> MRVVIVGGGFGGIAAASQLKSWAVPFVLVDMRDAFHHNVAALRASVESGFARKTFISYSVTFGDSFRQGKVVGIDPERQQVLLSDGEELHYSHLILATGSDGPFPGKFNKVIDMESAIQTYEDMVKEIEKSERILVVGGGAAGVEMAAEIKTEYPAKEVTLIHSKIALADVELLQSVRQEVKEILLRKGVRLLLSEKVSNVENLTTNQFQKDMVVRTEKGTEVVVDMVVLCTGIKINSSAYATAFGDKLASNGALNVNKHLQLEGYDNIYAIGDCANLKEPKMAYHAELHANIVVSNIINSLTHKPLKTYQPGSLTFLLSMGKNDGVGQVKGYYVGHLLVTIAKSRDLFVSKSWKTMGQPMPSLEHHHHHH

Ferroptosis suppressor protein 1 (FSP1, also known as AIMF2, AMID or PRG3) is a recently identified glutathione-independent ferroptosis suppressor, but its underlying structural mechanism remains unknown. FSP1 is recently identified as a breakthrough owing to its unique ability to suppress ferroptosis by reducing ubiquinone to ubiquinol, or vitamin K to reduced hydroquinone (VKH2). The overall structure of cFSP1ΔN adopts a glutathione reductase-like fold and is also composed of three domains, a FAD-binding domain (FBD, residues 12–141, and 241–318) harboring a FAD molecule, a NAD(P)H-binding domain (NBD, residues 142–240) and a C-terminal domain (CTD, residues 319–373). Our work reveals that the homodimer of FSP1 is required for the formation of FAD- and ubiquinone-binding pockets, as well as the activity of NAD(P)H: ubiquinone oxidoreduction and ferroptosis suppression.

We report the crystal structures of cFSP1 (residues 12–373, hereafter named cFSP1ΔN) in its substrate-free and ubiquinone (CoQ1)-bound forms at 2.0 and 2.6 Å resolution, respectively. The structure of the ubiquinone-bound form was obtained by co-crystallizing cFSP1ΔN with ubiquinone Q1 (CoQ1) in the absence of NAD(P)H. In both substrate-free and CoQ1-bound structures, each asymmetric unit contains one cFSP1ΔN molecule, and their structures are virtually identical (r.m.s. deviation of ~0.4 Å), with the exception of a loop 327–337 at CTD, which assumes two different conformations even though it is partially disordered and displays weak density, suggesting a role in regulating substrate access to the active site. The peteridine moiety of the isoalloxazine ring is located in a canonical active site for ubiquinone substrate binding (hereafter named ubiquinone-binding pocket), which is mainly formed by residues 293–298 of α10, residues 327–331 and 354–362 from CTD, residues 340–350 from CTD of the other chain in the dimer, where one CoQ1 molecule is clearly buried in. The CoQ1 interacts with cFSP1 by mainly hydrophobic interactions with residues forming the ubiquinone-binding pocket, including Ala294, Tyr295, residues 327–329, Phe359, Lys362 and two residues (Val340 and Leu348) from the other chain of the dimer. Moreover, the head group of CoQ1 interacts with the FAD through a hydrogen bond between the O4 atom of CoQ1 and N3 atoms of FAD. The mutation of Leu329 (Leu330 in hFSP1), which is positioned at the entrance loop for the substrate CoQ1, probably reduces the binding activity to CoQ. Notably, in these two structures, cFSP1ΔN molecule forms a dimer with its crystallographic symmetric molecule. The interactions between the two cFSP1 monomers are mainly mediated through its CTD.>SNAMRVIDTHCDALYKLQAGKGKYTFQDAEELDVNFERLIEAKMLLQGFAIFLDEDIPVEHKWKKAVEQVNIFKQHVLHKGGIIHHVKKWCDLENLPEDKIGAMLTLEGIEPIGRDLDKLTQLLDGGVLSVGLTWNNANLAADGIMEERGAGLTRFGKDIIHLLNERKVFTDVSHLSVKAFWETLEQAEFVIASHSSAKAICAHPRNLDDEQIKAMIEHDAMIHVIFH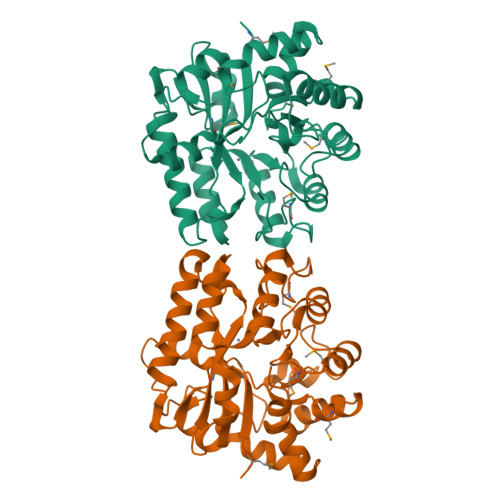PLFTTNDGVADIEDVIRHIDHICELGGMKNIGFGSDFDGIPDHVKGLEHAGKYQNFLETLGKHYTKEEVEGFASRNFLNHLPK[2x]> I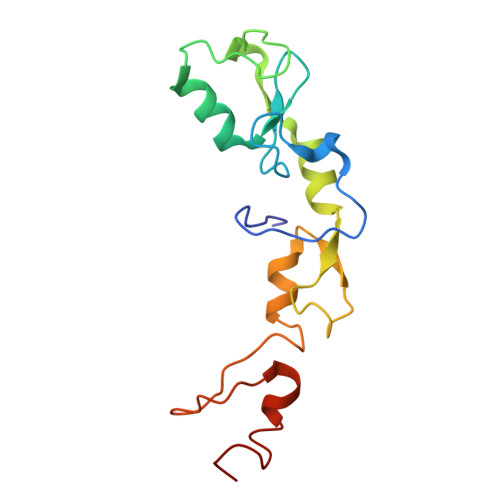SLDFEPSIEYQFVERLEERYKCAFCHSVLHNPHQTGCGHRFCQHCILSLRELNTVPICPVDKEVIKSQEVFKDNCCKREVLNLYVYCSNAPGCNAKVILGRYQDHLQQCLFQPVQCSNEKCREPVLRKDLKEHLSASCQFR> MGHHHHHHHHHHGNVQDALLTNQLYKNHELLKLERKKTEAVARLKSMNKSAINQYNRRQDKKNKRLKFGHRLIATHTNLERDEQKRAEKKAKERL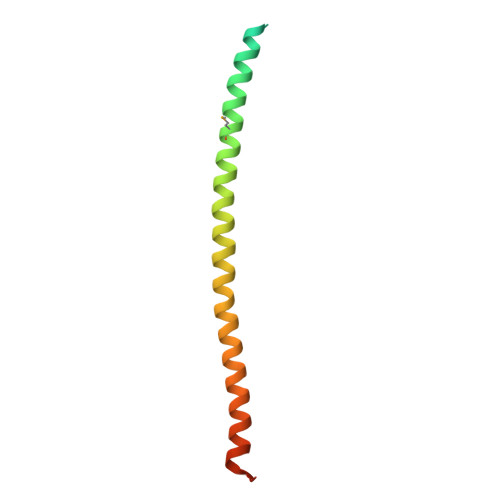QALKANDEEAY(2S)-N-methyl-N-{6-methyl-2-[(4aS,5aR)-5a-methyl-1,4,4a,5,5a,6-hexahydrocyclopropa[f]indazol-3-yl]-1H-1,3-benzimidazol-5-yl}-2-(morpholin-4-yl)propanamide 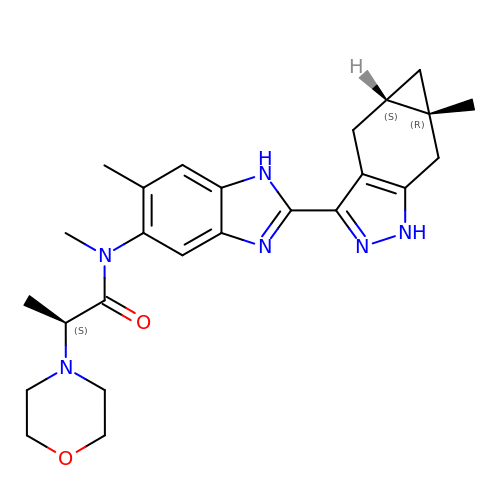| C25 H32 N6 O2 | DVXKDRBZBOJVGG-JAUXOLPYSA-N>MDYRQLHRWDLPPEEAIKVQNELRKKIKLTPYEGEPEYVAGVDLSFPGKEEGLAVIVVLEYPSFKILEVVSERGEITFPYIPGLLAFRQGPLFLKAWEKLRTKPDVVVFDGQGLAHPRKLGIASHMGLFIEIPTIGVAKSRLYGTFKMPEDKRC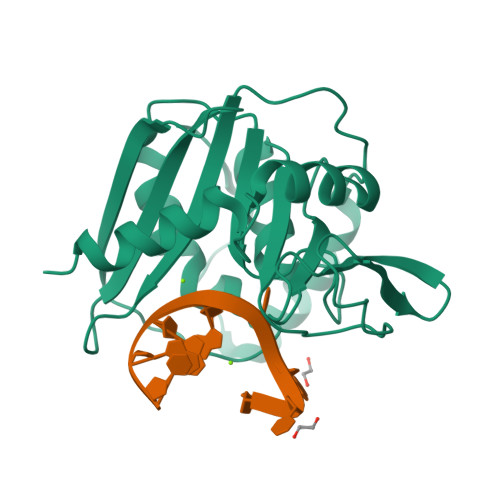SWSYLYDGEEIIGCVIRTKEGSAPIFVSPGHLMDVESSKRLIKAFTLPGRRIPEPTRLAHIYTQRLKKGL[2x]> VDCSEYPKPACTGEYRPLCGSDNKTYGNKCNFCNAVVESNGTLTLSHFG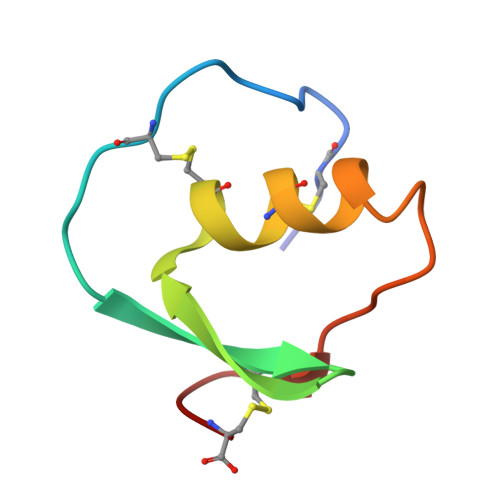KC> GLGPLQIWQTNFTLEPRMAPRSWLAVTVDTASSAIVVTQHGRVTSVAAQHHWATAIAVLGRPKAIKTDNGSCFTSKSTREWL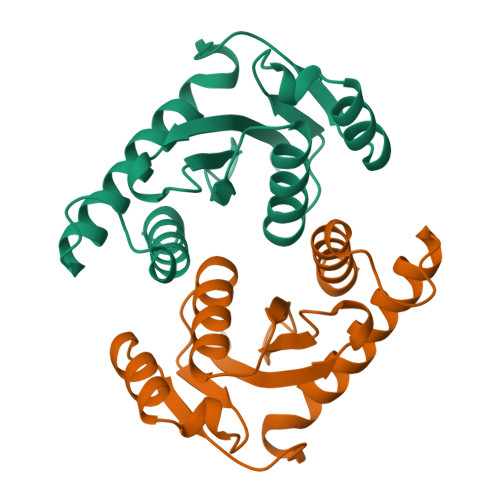ARWGIAHTTGIPGNSQGQAMVERANRLLKDKIRVLAEGDGFMKRIPTSKQGELLAKAMYALNHF>VQPLARDAMAYVLAGGRGSRLKELTDRRAKPAVYFGGKARIIDFALSNALNSGIRRIGVATAYKAHSLIRHLQRGWDFFRPERNESFDILPASQRVSETQWYEGTADAVYQNIDIIEPYAPEYMVILAGDHIYKMDYEYMLQQHVDSGADVTIGCLEVPRMEATGFGVMHVNEKDEIIDFIEKPADPPGIPGNEGFALASMGIYVFHTKFLMEALRRDAADPTSSRDFGKDIIPYIVEHGKAVAHRFADSCVRSDFEHEPYWRDVGTIDAYWQANIDLTDVVPDLDIYDKSWPIWTYAEITPPAKFVHDDEDRRGSAVSSVVSGDCIISGAALNRSLLFTGVRANSYSRLENAVVLPSVKIGRHAQLSNVVIDHGVVIPEGLIVGEDPELDAKRFRRTESGICLITQS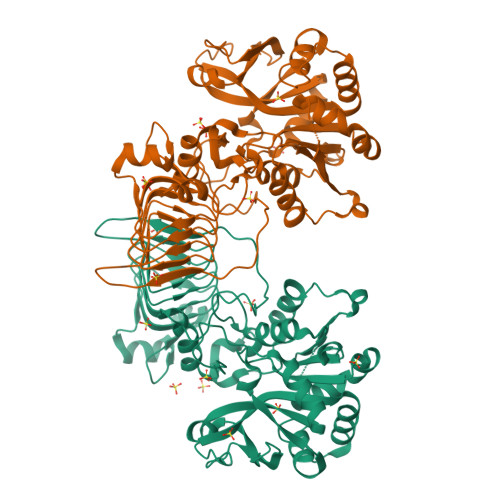MIDKL[10x]>MAYPDANLLNDRVLRAMLKAEETCAPSVSYFKCVQKEVLPSMRKIVATWMLEVCEEQKCEEEVFPLAMNYLDRFLS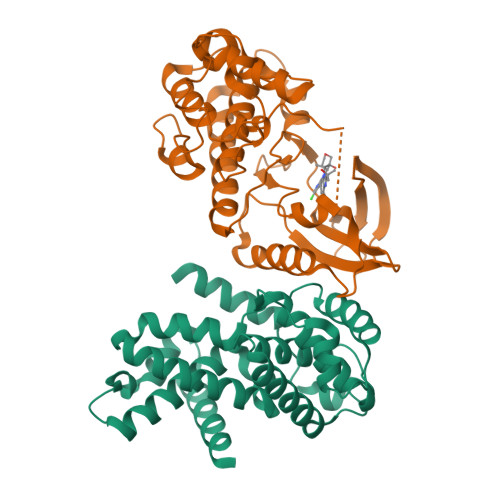LEPVKKSRLQLLGATCMFVASKMKETIPLTAEKLCIYTDNSIRPEELLQMELLLVNKLKWNLAAMTPHDFIEHFLSKMPEAEENKQIIRKHAQTFVALCATDVKFISNPPSMVAAGSVVAAVQGLNLRSPNNFLSYYRLTRFLSRVIKCDPDCLRACQEQIEALLESSLRQAQQNMDPKAA[2x];>[2x]MATSRYEPVAEIGVGAYGTVYKARDPHSGHFVALKSVRVPNGEEGLPISTVREVALLRRLEAFEHPNVVRLMDVCATSRTDREIKVTLVFEHVDQDLRTYLDKAPPPGLPAETIKDLMRQFLRGLDFLHANCIVHRDLKPENILVTSGGTVKLADFGLARIYSYQMALTPVVVTLWYRAPEVLLQSTYATPVDMWSVGCIFAEMFRRKPLFCGNSEADQLGKIFDLIGLPPEDDWPRDVSLPRGAFPPRGPRPVQSVVPEMEESGAQLLLEMLTFNPHKRISAFRALQHSYLHKDEGNPELENLYFQGHHHHHH> ADPLSVAADKLAKLERDFGGSIGVYAIDTGSGATVANRPNERFPLCSSFKGFLAAGVLAQSQDKPGLLDKRIRYSKAALPNWSPITTKHQASGMTVAELNAASVQYSDNGAANLLLKEINGPAALTTFMRSIGDASFRLDRLEPELNSAIPRDPRDTSTPKAVAESAQKLALGKALPEPQRQQLADWLKGNTTGNARIRA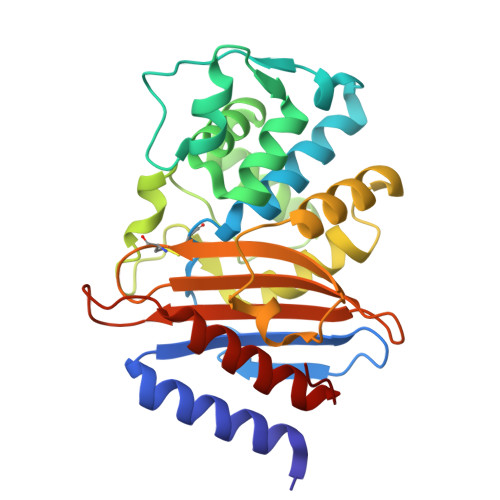AVPAGWEVGDKTGTCGVYGTANDFAVIWPPKRAPIVLAVYTKHAKKEAKHSDEVIAAAARAALEAFNVKK>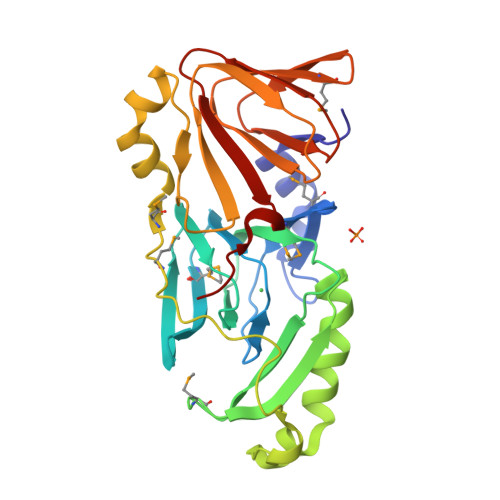 SERRLGVRAWVKENRGSFQPPVCNKLMHQEQLKVMFIGGPNTRKDYHIEEGEEVFYQLEGDMVLRVLEQGKHRDVVIRQGEIFLLPARVPHSPQRFANTVGLVVERRRLETELDGLRYYVGDTMDVLFEKWFYCKDLGTQLAPIIQEFFSSEQYRTGKPIPDQLLKEPPFPLSTRSIMEPMSLDAWLDSHHRELQAGTPLSLFGDTYETQVIAYGQGSSEGLRQNVDVWLWQLEGSSVVTMGGRRLSLAPDDSLLVLAGTSYAWERTQGSVALSVTQDPACKKPLG>[2x]GPKTLKFMTASSPLSPKDPNEKLILQRLEKETGVHIDWTNYQSDFAEKRNLDISSGDLPDAIHNDGASDVDLMNWAKKGVIIPVEDLIDKYMPNLKKILDEKPEYKALMTAPDGHIYSFPWIEELGDGKESIHSVNDMAWINKDWLKKLGLEMPKTTDDLIKVLEAFKNGDPNGNGE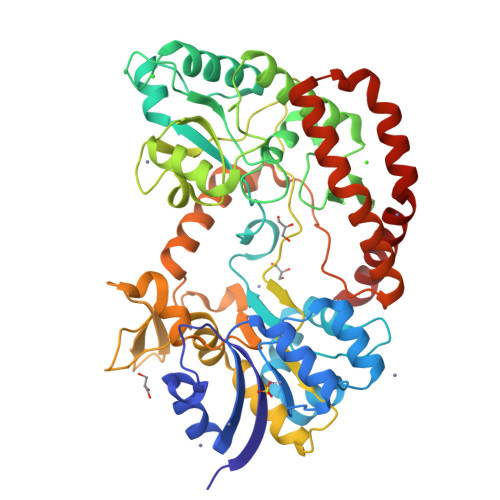ADEIPFSFISGNGNEDFKFLFAAFGIGDNDDHLVVGNDGKVDFTADNDNYKEGVKFIRQLQEKGLIDKEAFEHDWNSYIAKGHDQKFGVYFTWDKNNVTGSNESYDVLPVLAGPSGQKHVARTNGMGFARDKMVITSVNKNLELTAKWIDAQYAPLQSVQNNWGTYGDDKQQNIFELDQASNSLKHLPLNGTAPAELRQKTEVGGPLAILDSYYGKVTTMPDDAKWRLDLIKEYYVPYMSNVNNYPRVFMTQEDLDKIAHIEADMNDYIYRKRAEWIVNGNIDTEWDDYKKELEKYGLSDYLAIKQKYYDQYQANKN>MVLKVYGPHFASPKRALVTLIEKGVAFETIPVDLMKGEHKQPAYLALQPFGTVPAVVDGDYKIFESRAVMRYVAEKYRSQGPDLLGKTVEDRGQVEQWLDVEATTYHPPLLNLTLHIMFASVMGFPSDEKLIKESEEKLAGVLDVYEAHLSKSKYLAGDFVSLADLAH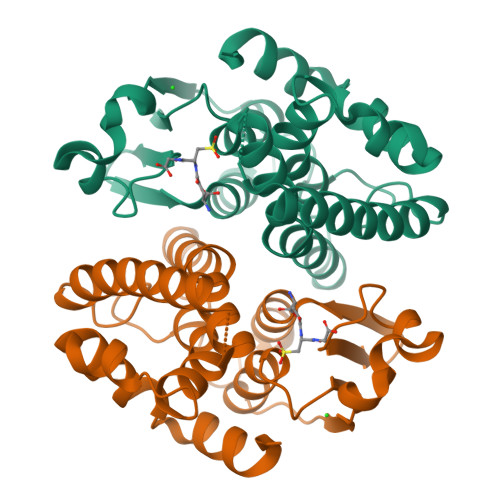LPFTDYLVGPIGKAYMIKDRKHVSAWWDDISSRPAWKETVAKYSFPA[10x]> DRWGSEILAETHGTRPDLTDQP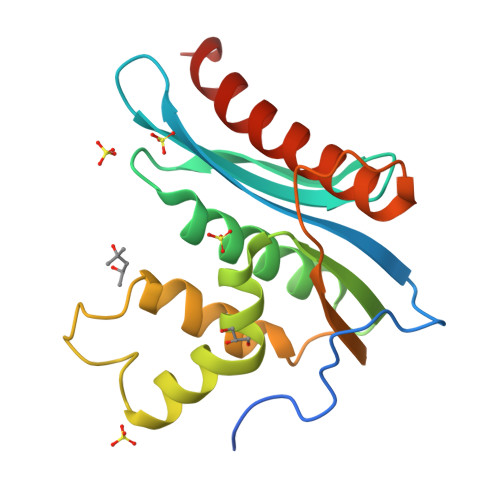IPDADYTWYTDGSSFLQEGQRRAGAAVTTETEVIWARALPAGTSAQRAELIALTQALKMAEGKKLNVYTDSRYAFATAHVHGEIYRRRGLLTSEGREIKNKNEILALLKALFLPKRLSIIHCPGHQKGNSAEARGNRMADQAAREAAMKAVLETSTLL>GPLGSDLKDAEAVQKFFLEEIQLGEELLAQGDYEKGVDHLTNAIAVSGQPQQLLQVLQQTLPPPV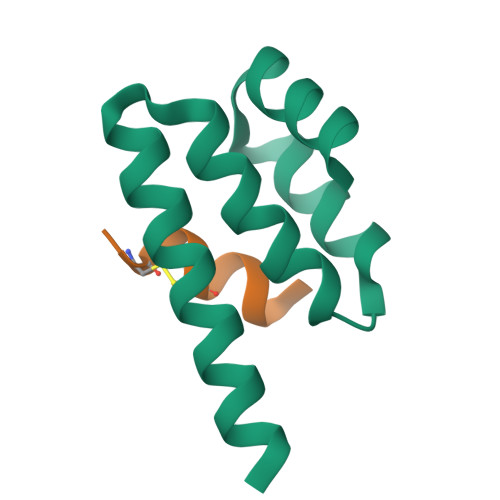FQMLLTKL[4x];>[4x]GCRLCRLLSYAX>MSSRPQREKSMTALTQHAPVLEIYQDIANLTSRMLAAANASNWDLVLNHGQEYVCLVERLRELEPGEPLDEAARGMKFDLLVRI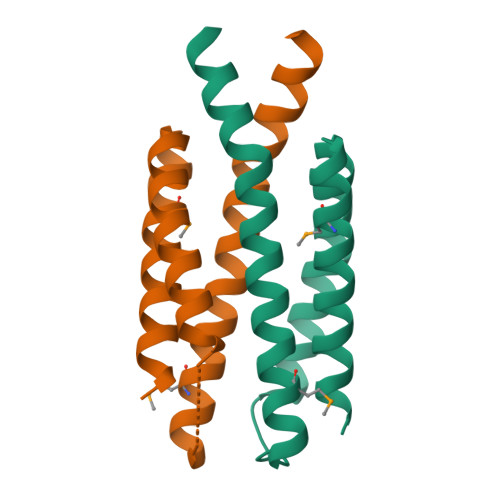LENDAAVRDLALPQLARLSDLLGRMKRQQSLLATYSGKANGT[2x]>[2x]MGKKIIALILIISTAIFGALYMYRNIFSFKDDNNIVALTKGKLISDVYTDKARYYPSDKVTVKIELNNELQEDFRGTIYIFYKHLESIVGKAKIQVNIKSGQKKQLNIFWEAPKDDFKGYLVEVYAVKGNKAIDNKNTAVDVSSDWSKFPRYGYI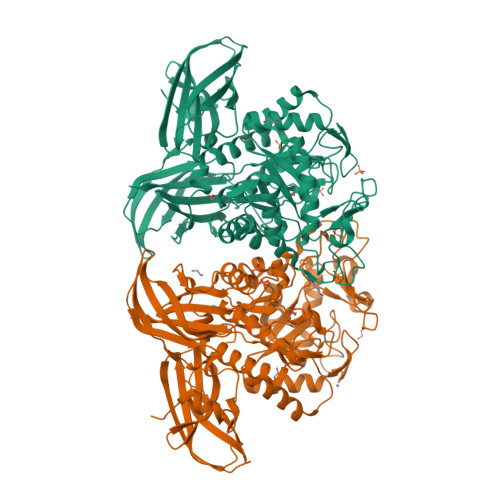ANFPEQSKEKSALIIEDLNKYHLNGLLFYDWQYKHNKPLAGTVENPDPKWKDIANRDIYGQTVKDYIELAHSKNIMVANYNLMYGGYFDYVKDGAKPEWGLYKDPNHEEQDNHPLPHTWATDRLYLFNPANKDWQNYIFNAEKDAFRVYNFDVWHVDTLGPRGMVYDYNGNPVELSFTYADFLNNAKNALGKRIVCNTVNEYGLINVASGADVDFLYVEIWPPARAHYNFLKQTVDNGYNYSDGKKATVVAAYMNYGIADRSAEFNKHSVRLTDAAIFAAGGDHIELGDTGMLSKEYFPSANLKMSESLVKAMRNYYDFLTAYENLLRDGLKESDNKIEIPGIEISNNGSARTVWTYAKQKDGYDVIHMINLLGIEVSNWRDDLGNYSAPPIIKDFKVKYYLENDNIKNVYLASPDINDGKVMKLQFKKKEDSKGKYLEISVPELQYWDMIFIKKLEHHHHHH>MSTVATYSYTHSVTYVTDNILKSLKDIILLSGLDPEHFADRWESNTRAIKTWLGTGDLRKVILEIYNPATDKLVTRWDIDIVYGWSDGDGSFWTDTEQLKYAIKKAG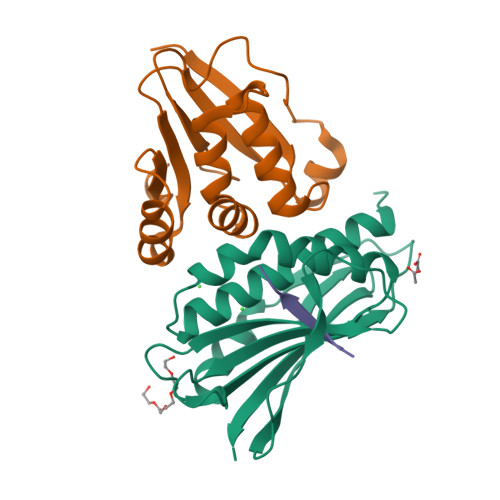LLPSQAKYKLMLDTKPGRPDVEGWSKGSYRSTDGMVKQSLGSTVEHSGLAGQAGYWRQR[2x];>[2x]MTTVVSRTFRSSPHRDALQTWDAIVELLTQGKDGTARSELRAVTGVAASLIADQAPKSAPIVATCDGPRTRIYCLFDEDAIDGDDANEEVLGFEPLKGDWGVSLPCPKEQLGWVQSALKKHSSRIIARDLSQG;>[2x]SNAEVMEFNP> KETAAAKFERQHMDSSTSAASSSNYCNQMMKSRNLTKDRCKPVNTFVHESLADVQAVCSQKNVACKNGQTNCYQSYSTMSITDCRETGSSKYPNCAYKT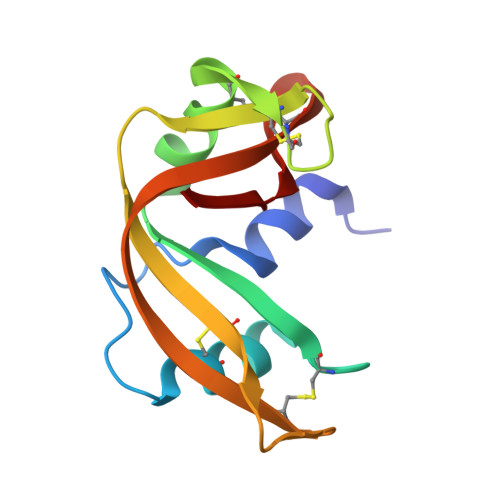TQANKHIIVACEGNPYVPVHFNASV2-(3-methoxyphenyl)-N-[4-(pyridin-4-yl)-1,3-thiazol-2-yl]acetamide 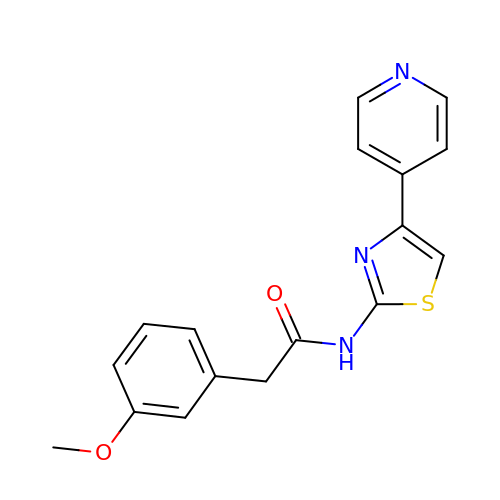| C17 H15 N3 O2 S | GOPDRFODUBCWMB-UHFFFAOYSA-N>[2x]SNAMKELIKVIAFDADDTLWSNEPFFQEVEKQYTDLLKPYGTSKEISAALFQTEMNNLQILGYGAKAFTISMVETALQISNGKIAADIIRQIVDLGKSLLKMPIELLPGVKETLKTLKE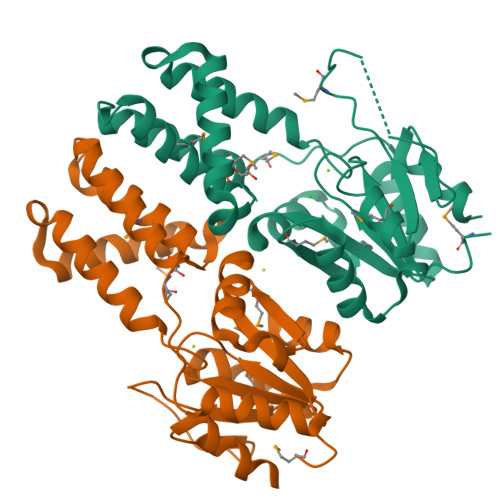TGKYKLVVATKGDLLDQENKLERSGLSPYFDHIEVMSDKTEKEYLRLLSILQIAPSELLMVGNSFKSDIQPVLSLGGYGVHIPFEVMWKHEVTETFAHERLKQVKRLDDLLSLLG4-METHYLPYRIDIN-2-AMINE | C6 H8 N2 | 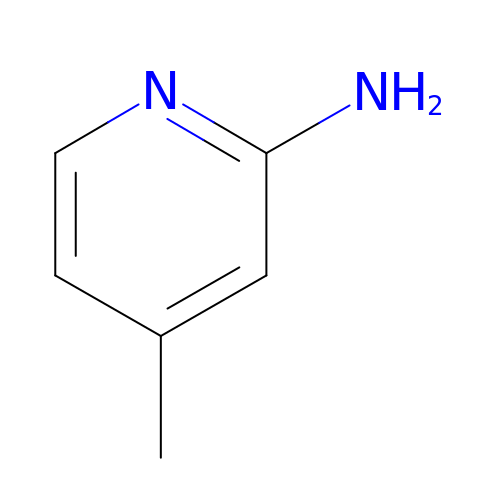ORLGLBZRQYOWNA-UHFFFAOYSA-N>[2x]SEDYERRRSECVSE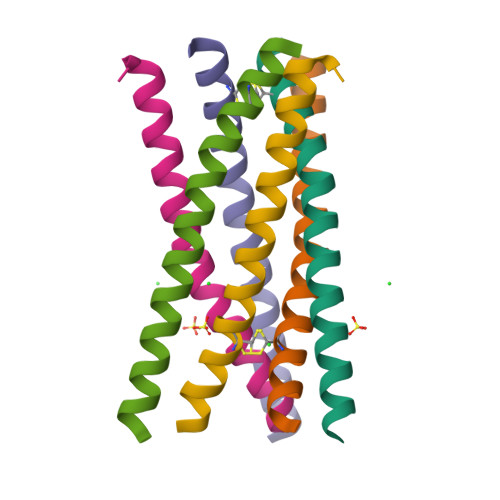MLDLEKQFSELKEKLFRERLSQLRLRLEEVGAERA> ELPQMTQQLNSDDMQEQLSATVKFRQILSREHRPPIDVVIQAGVVPRLVEFMRENQPEMLQLEAAWALTNIASGTSAQTKVVVDADAVPLFIQLLYTGSVEVKEQAIWALGNVAGDSTDYRDYVLQCNAMEPILGLFNSNKPSLIRTATWTLSNLCRGKKPQPDWSVVSQALPTLAKLIYSMDTETLVDACWAISYLSDGPQEAIQAVIDVRIPKRLVELLSHESTLVQTPALRAVGNIVTGNDLQTQVVINAGVLPALRLLLSSPKENIKKEACWTISNITAGNTEQIQAVIDANLIPPLVKLLEVAEDKTKKEACWAISNASSGGLQRPDIIRYLVSQGCIKPLCDLLEIADNRIIEVTLDALENILKMGEADKEARGLNINENADFIEKAGGMEKIFNCQQNEND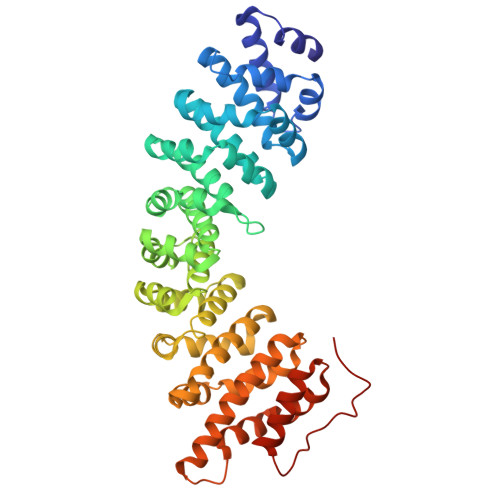KIYEKAYKIIETYFGEEEDAVDETMAPQNAGNTFG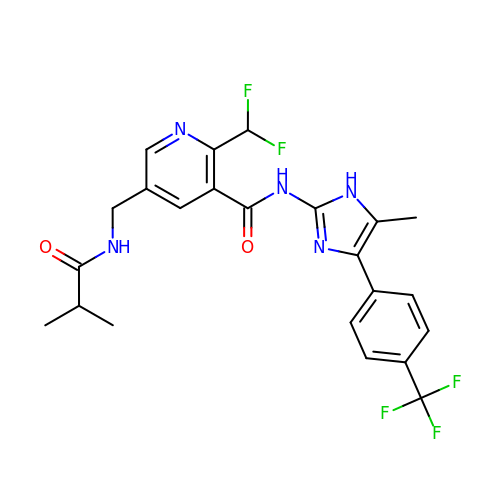2-(difluoromethyl)-5-{[(2-methylpropanoyl)amino]methyl}-N-{5-methyl-4-[4-(trifluoromethyl)phenyl]-1H-imidazol-2-yl}pyridine-3-carboxamide | C23 H22 F5 N5 O2 | BZYSILFNUIGABU-UHFFFAOYSA-N> MEEPFEAYRSREVAMKLVEKIREEAKTLDGEIRIMHVCGTHEDTVTRHGIRSLLPENVKVVSGPGCPVCITPVEDIVAMQLIMRKAREEGEE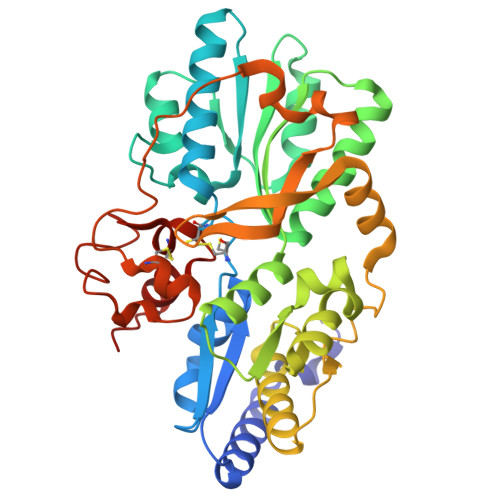IILTTFGDMYKIPTPMGSFADLKSEGFDVRIVYGIFDTYRIAKENPDKTVVHFSPGFETTTAPAAGMLNVAAQEELENFKIYSVHRLTPPAVEVLLKQGTVFQGLIAPGHVSTIIGVKGWEYLTEKYGIPQVVAGFEPNDVLMAILMLIRMYKEGEARIINEYERAVKYEGNVVAQKMIDKFFEVVDAKWRALGVFPKSGLELRKEWKDFEIRSFYKVEVPKNLPDLEKGCRCGAVLRGLALPTDCPLFGKTCTPRHPVGPCMVSYEGTCQIFYKYGVLF>[2x]GSQKERLLDELTLEGVARYMQSERCRRVICLVGAGISTSAGIPDFRSPSTGLYDNLEKYHLPYPEAIFEISYFKKHPEPFFALA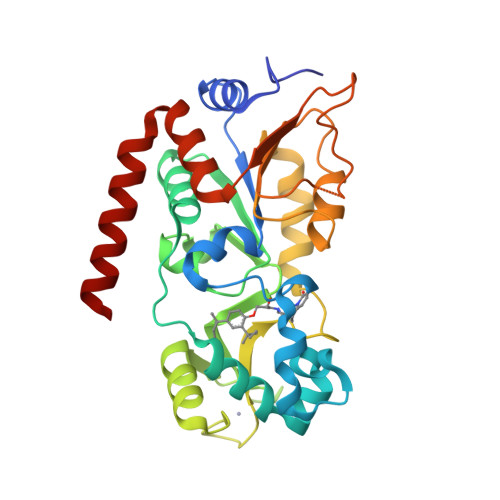KELYPGQFKPTICHYFMRLLKDKGLLLRCYTQNIDTLERIAGLEQEDLVEAHGTFYTSHCVSASCRHEYPLSWMKEKIFSEVTPKCEDCQSLVKPDIVFFGESLPARFFSCMQSDFLKVDLLLVMGTSLQVQPFASLISKAPLSTPRLLINKEKAGGGGMDFDSKKAYRDVAWLGECDQGCLALAELLGWKKELEDLVRREHASIDAQS Using an X-ray free electron laser (XFEL), we have previously determined room-temperature (RT) serial femtosecond crystallography (SFX) structures of the ferric and Compound I redox states of DtpB,26 a B-type member of the dye-decolorizing peroxidase (DyP) family. Such an approach results in “pristine” DtpB structures that do not exhibit the effects of X-ray-generated radiation damage. The RT-SFX DtpB ferric and Compound I structures revealed that the distal heme pocket, which is composed of an Asp–Arg–Asn triad, was void of H2O molecules. DtpB, therefore, represents an exemplar of a His–heme-ligated peroxidase in which the distal heme pocket favors a dry site. By disrupting the distal heme pocket Asp–Asn–Arg triad in DtpB, our RT-SFX structures reveal that a wet site can be formed.

To assess whether disruption of the Asp–Arg–Asn triad in DtpB leads to a wet distal heme pocket, microcrystals of each variant in the Fe(III)–heme state were produced and subjected to RT-SFX crystallography using a high viscosity extruder sample delivery system at the SACLA XFEL beamline BL2 EH3. For all variants, well-defined electron density peaks were present in the distal heme pocket, consistent with the presence of resident H2O molecules. In the N245A variant, only one resident H2O is found, and in the R243A variant, four resident H2O molecules are observed, with three of these accommodated within the distal pocket and the fourth positioned in the space vacated by the Arg243 side chain. This arrangement enables w1 to be directly linked through a H-bonding network to bulk H2O (wb in Figure 1). In the D152A, D152A/N245A, and R243 variants, w1 is positioned close enough to the heme–Fe(III) to be a bonding interaction (average Fe(III)–OH2 distances within the DtpB hexamer assembly of 2.52, 2.83, and 2.28 Å, respectively). Site-directed mutagenesis has revealed that distal Arg243, and not Asp152, facilitates proton movement on H2O2 binding to Fe(III)–heme, promoting the heterolysis of the O–O bond. We have previously reported that the distal heme pocket Arg243 and not Asp152 modulates the kinetics of Compound I formation upon mixing H2O2 with DtpB.

>[6x]EPEPQMVLSPLTSAAIFLVVTIDSGGEDTVRDLLSDVASLERAVGFRAQPDGRLSCVTGIGSEAWDRLFSGARPAGLHPFRELDGPVHRAVATPGDLLFHIRASRLDLCFALATEIMGRLRGAVTPQDEVHGFKYFDERDMLGFVDGTENPTGAAARRAVLVGAEDPAFAGGSYAVVQKYLHDIDAWEGLSVEAQERVIGRRKMTDVELSDDVKPADSHVALTSVTGPDGSDLEILADNMPFGSVGREEFGTYFIGYARTPEVTETMLERMFLGTASAPHDRILDFSTAVTGSLFFTPAADFLEDLS> MRALLPYLALYKRHKWMLSLGIVLAIVTLLASIGLLTLSGWFLSASAVAGVAGLYSFNYMLPAAGVRGAAITRTAGRYFERLVSHDATFRVLQHLRIYTFSKLLPLSPAGLARYR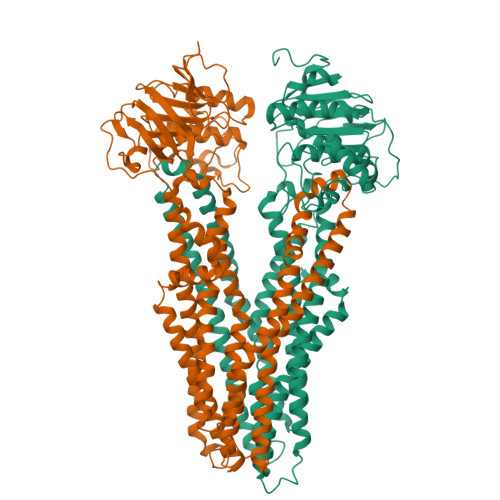QGELLNRVVADVDTLDHLYLRVISPLVGAFVVIMVVTIGLSFLDFTLAFTLGGIMLLTLFLMPPLFYRAGKSTGQNLTHLRGQYRQQLTAWLQGQAELTIFGASDRYRTQLENTEIQWLEAQRRQSELTALSQAIMLLIGALAVILMLWMASGGVGGNAQPGALIALFVFCALAAFEALAPVTGAFQHLGQVIASAVRISDLTDQKPEVTFPDTQTRVADRVSLTLRDVQFTYPEQSQQALKGISLQVNAGEHIAILGRTGCGKSTLLQQLTRAWDPQQGEILLNDSPIASLNEAALRQTISVVPQRVHLFSATLRDNLLLASPGSSDEALSEILRRVGLEKLLEDAGLNSWLGEGGRQLSGGELRRLAIARALLHDAPLVLLDQPTEGLDATTESQILELLAEMMREKTVLMVTHRLRGLSRFQQIIVMDNGQIIEQGTHAELLARQGRYYQFKQGL;> MNKSRQKELTRWLKQQSVISQRWLNISRLLGFVSGILIIAQAWFMARILQHMIMENIPREALLLPFTLLVLTFVLRAWVVWLRERVGYHAGQHIRFAIRRQVLDRLQQAGPAWIQGKPAGSWATLVLEQIDDMHDYYARYLPQMALAVSVPLLIVVAIFPSNWAAALILLGTAPLIPLFMALVGMGAADANRRNFLALARLSGHFLDRLRGMETLRIFGRGEAEIESIRSASEDFRQRTMEVLRLAFLSSGILEFFTSLSIALVAVYFGFSYLGELDFGHYDTGVTLAAGFLALILAPEFFQPLRDLGTFYHAKAQAVGAADSLKTFMETPLAHPQRGEAELASTDPVTIEAEELFITSPEGKTLAGPLNFTLPAGQRAVLVGRSGSGKSSLLNALSGFLSYQGSLRINGIELRDLSPESWRKHLSWVGQNPQLPAATLRDNVLLARPDASEQELQAALDNAWVSEFLPLLPQGVDTPVGDQAARLSVGQAQRVAVARALLNPCSLLLLDEPAASLDAHSEQRVMEALNAASLRQTTLMVTHQLEDLADWDVIWVMQDGRIIEQGRYAELSVAGGPFATLLAHRQEEI>GPNQDELKQLVGTKAVEWIKDGMIVGLGTGSTVKYMVDALGKRVNEEGLDIVGVTTSIRTAEQAKSLGIVIKDIDEVDHIDLTIDGADEISSDFQGIKGGGAALLYEKIVATKSNKNMWIVDESKMVDDLGQFPLPVEV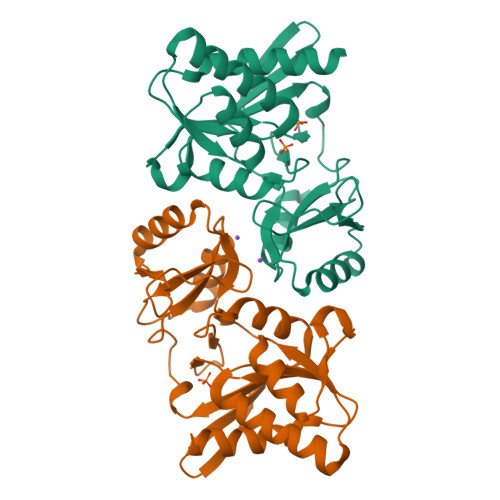IPYGSGTVFKRFEEKGLNPEFRKNEDGSLLHTDSDNYIIDLHLGKIENPKELGDYLINQVGVVEHGLFLDIVNTVIVGRQDGPEVLEAR[2x]>MRKFRLIPYKQVDKVSALSEVPMGVEIVEAPAVWRASAKGAGQIIGVIDTGCQVDHPDLAERIIGGVNLTTDYGGDETN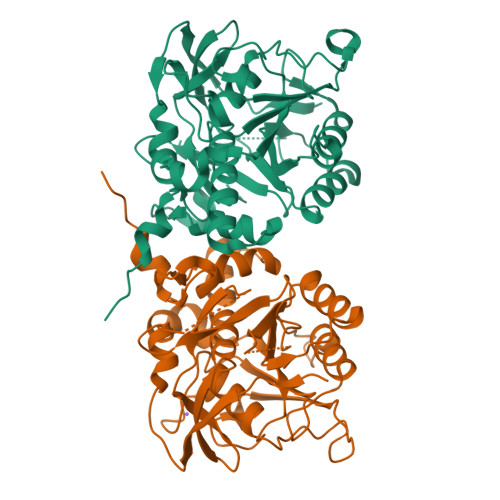FSDNNGHGTHVAGTVAAAETGSGVVGVAPKADLFIIKALSGDGSGEMGWIAKAIRYAVDWRGPKGEQMRIITMSLGGPTDSEELHDAVKYAVSNNVSVVCAAGNEGDGREDTNEFAYPAAYNEVIAVGAVDFDLRLSDFTNTNEEIDIVAPGVGIKSTYLDSGYAELSGTAMAAPHVAGALALIINLAEDAFKRSLSETEIYAQLVRRATPIGFTAQAEGNGFLTLDLVERITGQFTEKGKKLEHHHHHH[6x]1-[2-methyl-5-(2-piperazin-1-yl-1,3-thiazol-4-yl)-4-[3,3,3-tris(fluoranyl)propyl]-1~{H}-pyrrol-3-yl]ethanone | C17 H21 F3 N4 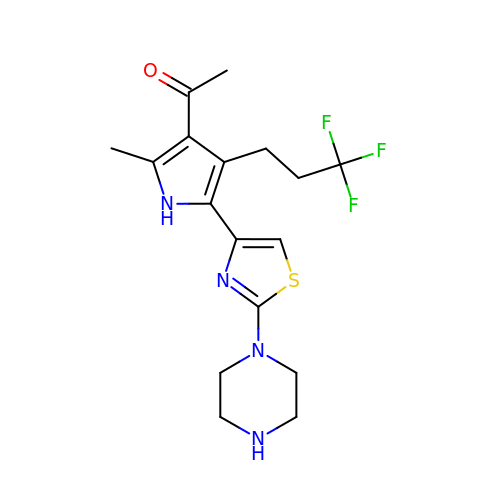O S | MWUAUINBVTULOI-UHFFFAOYSA-N(2~{R})-2-[(4~{S})-6-(4-chlorophenyl)-8-methoxy-1-methyl-4~{H}-[1,2,4]triazolo[4,3-a][1,4]benzodiazepin-4-yl]-~{N}-ethyl-propanamide 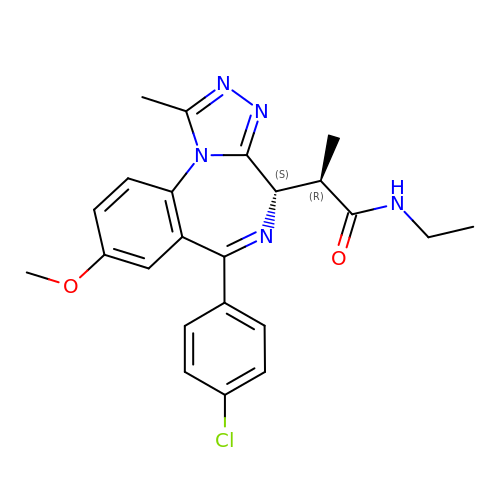| C23 H24 Cl N5 O2 | LTQHMHHEKFOBRX-XCLFUZPHSA-N> MPEPTADAPTVPKARSCPFLPPDGIADIRAAAPVTRATFTSGHEAWLVTGYEEVRALLRDSSFSVQVPHALHTQDGVVTQKPGRGSLLWQDEPEHTSDRKLLAKEFTVRRMQALRPNIQRIVDEHLDAIEA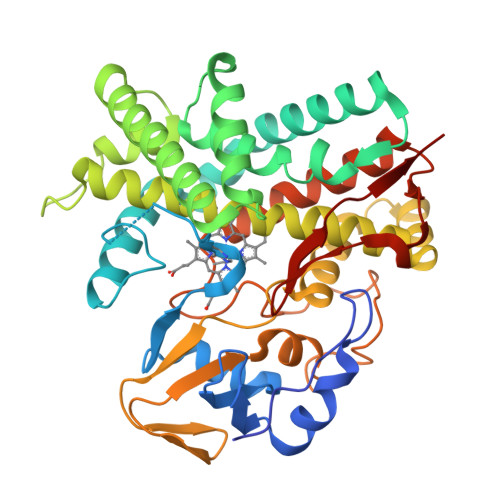RGGPVDLVKTFANAVPSMVISDLFGVPVERRAEFQDIAEAMMRVDQDAAATEAAGMRLGGLLYQLVQERRANPGDDLISALITTEDPDGVVDDMFLMNAAGTLLIAAHDTTACMIGLGTALLLDSPDQLALLREDPSLVGNAVEELLRYLTIGQFGGERVATRDVELGGVRIAKGEQVVAHVLAADFDPAFVEEPERFDITRRPAPHLAFGFGAHQCIGQQLARIELQIVFETLFRRLPGLRLAKPVEELRFRHDIVFYGVHELPVTWHHHH> MNSPISPIETVPVKLKPGMDG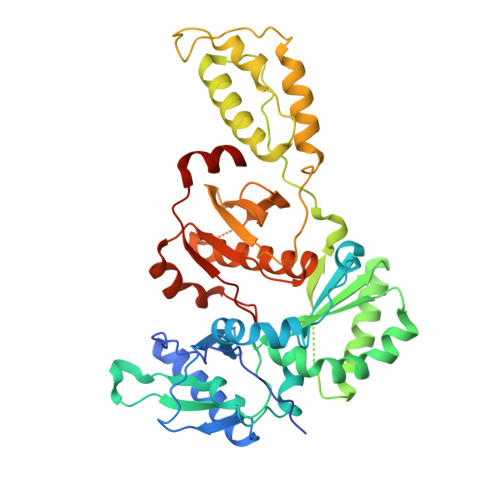PKVKQWPLTEEKIKALVEICTEMEKEGKISKIGPENPYNTPVFAIKKKDSTKWRKLVDFRELNKRTQDFWEVQLGIPHPAGLKKKKSVTVLDVGDAYFSVPLDEDFRKYTAFTIPSINNETPGIRYQYNVLPQGWKGSPAIFQSSMTKILEPFRKQNPDIVIYQYMDDLYVGSDLEIGQHRTKIEELRQHLLRWGLTTPDKKHQKEPPFLWMGYELHPDKWTVQPIVLPEKDSWTVNDIQKLVGKLNWASQIYPGIKVRQLCKLLRGTKALTEVIPLTEEAELELAENREILKEPVHGVYYDPSKDLIAEIQKQGQGQWTYQIYQEPFKNLKTGKYARMRGAHTNDVKQLTEAVQKITTESIVIWGKTPKFKLPIQKETWETWWTEYWQATWIPEWEFVNTPPLVKLWYQLEKEPIVGAETF>MADYKDDDDKGTDYKDDDDKLEVLFQGPMEANQCPLVVEPSYPDLVINVGEVTLGEENRKKLQKIQRDQEKERVMRAACALLNSGGGVIRMAKKVEHPVEMGLDLEQSLRELIQSSDLQAFFETKQQGRCFYIFVKSWSSGPFPEDRSVKPRLCSLSSSLYRRSETSVRSMDSREAFCFLKTKRKPKILEEGPFHKIHKGVYQELPNSDPADPNSDPADLIFQKDYLEYGEILPFPESQLVEFKQFSTKHFQEYVKRTIPEYVPAFANTGGGYLFIGVDDKSREVLGCAKENVDPDSLRRKIEQAIYKLPCVHFCQPQRPITFTLKIVNVLKRGELYGYACMIRVNPFCCAVFSEAPNSWIVEDKYVCSLTTEKWVGMMTDTDPDLLQLSEDFECQLSLSSGPPLSRPVYSKKGLEHKKELQQLLFSVPPGYLRYTPESLWRDLISEHRGLEELINKQMQPFFRGILIFSRSWAVDLNLQEKPGVICDALLIAQNSTPILYTILREQDAEGQDYCTRTAFTLKQKLVNMGGYTGKVCVRAKVLCLSPESSAEALEAAVSPMDYPASYSLAGTQHMEALL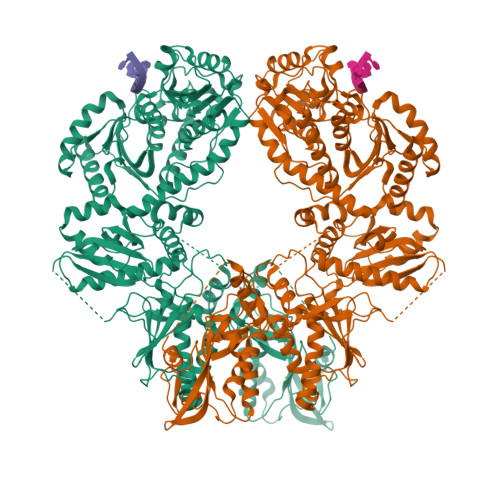QSLVIVLLGFRSLLSDQLGCEVLNLLTAQQYEIFSRSLRKNRELFVHGLPGSGKTIMAMKIMEKIRNVFHCEAHRILYVCENQPLRNFISDRNICRAETRKTFLRENFEHIQHIVIDEAQNFRTEDGDWYGKAKSITRRAKGGPGILWIFLDYFQTSHLDCSGLPPLSDQYPREELTRIVRNADPIAKYLQKEMQVIRSNPSFNIPTGCLEVFPEAEWSQGVQGTLRIKKYLTVEQIMTCVADTCRRFFDRGYSPKDVAVLVSTAKEVEHYKYELLKAMRKKRVVQLSDACDMLGDHIVLDSVRRFSGLERSIVFGIHPRTADPAILPNVLICLASRAKQHLYIFPWGGH[2x]> MSKAKIGIVTVSDRASAGITADISGKAIILALNLYLTSEWEPIYQVIPDEQKVIERTLIKMADIQDCCLIVTTGGTGPAKRDVTPEATEAVCD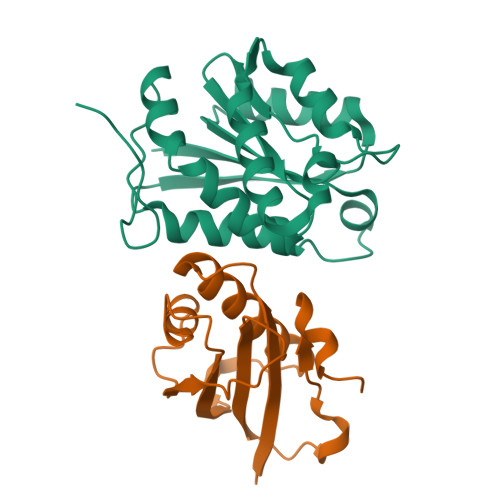RMMPGFGELMRAESLKEVPTAILSRQTAGLRGDSLIVNLPGDPASISDCLLAVFPAIPYCIDLMEGPYLECNEAMIKPFRPKAKLEHHHHHH;> MVRGIRGAITVNSDTPTSIIIATILLLEKMLEANGIQSYEELAAVIFTVTEDLTSAFPAEAARQIGMHRVPLLSAREVPVPGSLPRVIRVLALWNTDTPQDRVRHVYLSEAVRLRPDLESAQLEHHHHHH>[3x]MTYGGRDQQYNKTNYKSRGGDFRGGRNSDRNSYNDRPQGGNYRGGFGGRSNYNQPQELIKPNWDEELPKLPTFEKNFYVEHESVRDRSDSEIAQFRKENEMTISGHDIPKPITTFDEAGFPDYVLNEVKAEGFDKPTGIQCQGWPMALSGRDMVGIAATGSGKTLSYCLPGIVHINAQPLLAPGDGPIVLVLAPTRELAVQIQTECSKFGHSSRIRNTCVYGGVPKSQQIRDLSRGSEIVIATPGRLIDMLEIGKTNLKRVTYLVLDEADRMLDMGFEPQIRKIVDQIRPDRQTLMWSATWPKEVKQLAADYLNDPIQVQVGSLELSASHNITQIVEVVSDFEKRDRLNKYLETASQDNEYKTLIFASTKRMCDDITKYLREDGWPALAIHGDKDQRERDWVLQEFRNGRSPIMVATDVAARGID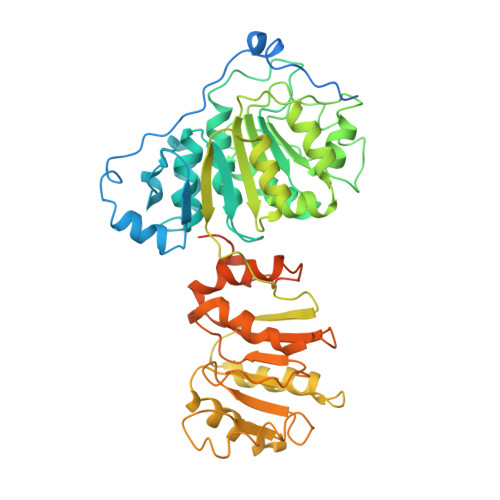VKGINYVINYDMPGNIEDYVHRIGRTGRAGATGTAISFFTEQNKGLGAKLISIMREANQNIPPELLKYDRRSYGGGHPRYGGGRGGRGGYGRRGGYGGGRGGYGGNRQRDGGWGNRGRSNY>MEGLAGY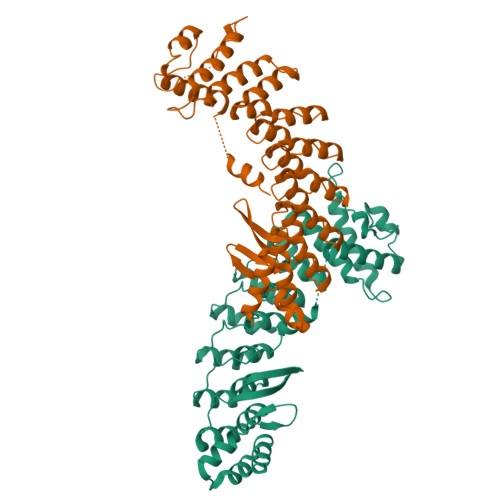VYKAASEGKVLTLAALLLNRSESDIRYLLGYVSQQGGQRSTPLIIAARNGHAKVVRLLLEHYRVQTQQTGTVRFDGYVIDGATALWCAAGAGHFEVVKLLVSHGANVNHTTVTNSTPLRAACFDGRLDIVKYLVENNANISIANKYDNTCLMIAAYKGHTDVVRYLLEQRADPNAKAHCGATALHFAAEAGHIDIVKELIKWRAAIVVNGHGMTPLKVAAESCKADVVELLLSHADCDRRSRIEALELLGASFANDRENYDIIKTYHYLYLAMLERFQDGDNILEKEVLPPIHAYGNRTECRNPQELESIRQDRDALHMEGLIVRERILGGGGSGGGSGSQKWKLIGLQR[2x]Recently, a new SAM-riboswitch class, termed SAM-VI, has been identified in species of Bifidobacterium by Breaker and co-workers using computational methods of comparative sequence analysis. One transcript from B. angulatum 59 metK in which the U1A recognition site had been introduced as terminal loop of stem P2 (and the non-conserved G42 had been mutated to U42) yielded diffraction quality crystals when co-crystallized with the U1A protein. The SAM-VI fold is composed of three stems P1, P2, and P3 that are consistent with the originally predicted secondary structure. Stem P2 (in violet) stacks co-axially with stem P1 (in green), mediated by two intercalating base pairs from the junctional region of the riboswitch and the ligand SAM.

We solved the structure with single-wavelength anomalous diffraction (SAD) phasing by collecting the anomalous signal of selenium in selenomethionine (SeMet)-derivatized U1A protein used in co-crystallization. The surface representation of the SAM-VI pocket shows that the adenine base of SAM (shown in sticks) is intercalating and becomes stacked, while the sulfonium moiety and the methionine tail point outward from the adenine intercalation site. The binding pocket itself is composed of one terminal Watson-Crick base pair G9-C32 from stem P2, one non-canonical (trans Watson-Crick) base pair G7•G33 from J1-2 and J2-3, four continuously stacked residues A34, A36, A37, and G38 from J2-3, and importantly, the U8 (from J1-2) that recognizes the SAM-adenine base. The SAM ligand adopts a C3′-endo ribose conformation and the SAM-adenine base is in anti conformation at the glycosidic bond when bound to SAM-VI RNA. The Hoogsteen edge of the SAM-adenine pairs with the Watson-Crick edge of U8. Furthermore, 6-NH2 of A36 and N1 of A37 also form one hydrogen bond each with the Watson-Crick edge of the adenine base of SAM. The non-bridging phosphate-oxygen of G33 forms one hydrogen bond with the 2′-OH of the ribose sugar of SAM. Notably, the methionine tail is structured and folds back, supported by an H-bond interaction between the α-amino group of the SAM methionine and O4 of U8. We further note that the sulfonium moiety of SAM is in the vicinity of the O4 atom of the U6 nucleobase (4.8 Å). The O4 of U6 likely assists in recognition and stabilization of the positive charge of the sulfonium moiety.

>[3x]TRPNHTIYINNLNEKIKKDELKKSLHAIFSRFGQILDILVKRSLKMRGQAFVIFKEVSSATNALRSMQGFPFYDKPMRIQYAKTDSDIIAKMA>[2x]QFTDIDKLAVSTIRILAVDTVSKANSGHPGAPLGMAPAAHVLWSQMRMNPTNPDWINRDRFVLSNGHAVALLYSMLHLTGYDLSIEDLKQFRQLGSRTPGHPEFELPGVEVTTGPLGQGISNAVGMAMAQANLAATYNKPGFTLSDNYTYVFLGDGCLQEGISSEASSLAGHLKLGNLIAIYDDNKITIDGATSISFDEDVAKRYEAYGWEVLYVENGNEDLAGIAKAIAQAKLSKDKPTLIKMTTTIGYGSLHAGSHSVHGAPLKADDVKQLKSKFGFNPDKSFVVPQEVYDHYQKTILKPGVEANNKWNKLFSEYQKKFPELGAELARRLSGQLPANWESKLPTYTAKDSAVATRKLSETVLEDVYNQLPELIGGSADLTPSNLTRWKEALDF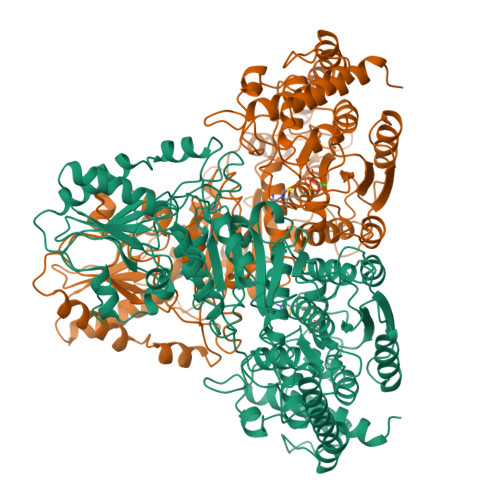QPPSSGSGNYSGRYIRYGIREHAMGAIMNGISAFGANYKPYGGTFLNFVSYAAGAVRLSALSGHPVIWVATHDSIGVGEDGPTHQPIETLAHFRSLPNIQVWRPADGNEVSAAYKNSLESKHTPSIIALSRQNLPQLEGSSIESASKGGYVLQDVANPDIILVATGSEVSLSVEAAKTLAAKNIKARVVSLPDFFTFDKQPLEYRLSVLPDNVPIMSVEVLATTCWGKYAHQSFGIDRFGASGKAPEVFKFFGFTPEGVAERAQKTIAFYKGDKLISPLKKAF>GSHHPFTAQIVAVTASGYDSEKGHVPANIADGDVKTRWAASGESWVQLELDKEQSI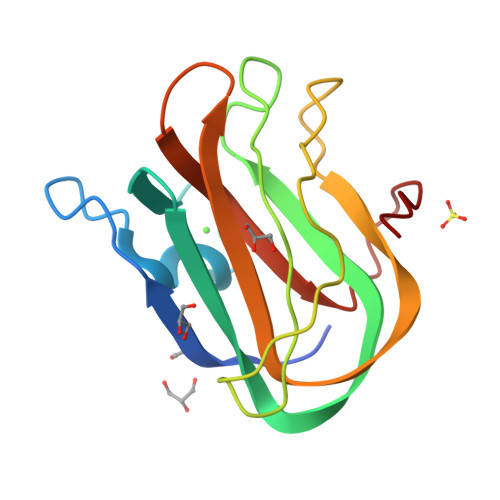ENILIVPFKPTERKLKFSIFYSNDGKNWQPLAEGLETSSADKNGEKLTFTPVTAKYIKLDTFGTDVNNWSAINEIAINSAAALPSRAIK[2x]>[2x]STAGKVIKCKAAVLWEEKKPFSIEEVEVAPPKAHEVRIKMVATGICRSDDHVVSGTLVTPLPVIAGHEAAGIVESIGEGVTTVRPGDKVIPLFTPQCGKCRVCKHPEGNFCLKNDLSMPRGTMQDGTSRFTCRGKPIHHFLGTSTFSQYTVVDEISVAKIDAASPLEKVCLIACGFSTGYGSA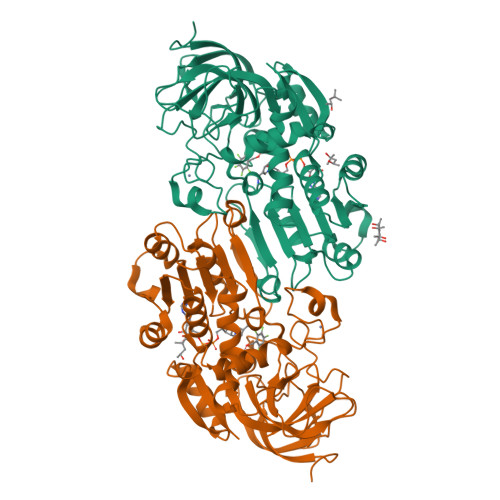VKVAKVTQGSTCAVFGLGGVGLSVIMGCKAAGAARIIGVDINKDKFAKAKEVGATECVNPQDYKKPIQEVLTEMSNGGVDFSFEVIGRLDTMVTALSCCQEAYGVSVIVGVPPDSQNLSMNPMLLLSGRTWKGAIFGGFKSKDSVPKLVADFMAKKFALDPLITHVLPFEKINEGFDLLRSGESIRTILTF> ANVWGVRLADSLSSPTIETRTRQYTLHDLCSDLDANPGREPWKPLRNQRTNNIVAVQLFRPLQGLVLDTQLYGFPGAFDDWERFMREKLRVLKYEVLRIYPISNYSNEHVNVFVANALVGAFLSNQAFYDLLPLLIINDTMIGDLLGTGASLSQFFQSHGDVLEVAAGRKYLQMENYSNDDDDPPLFAKDLSDYAKAFYSDTYEVLDRFFWTHDSSAGVLVHYDKPTNGHHYLLGTLTQMVSAPPYIINATDAMLLESCLEQFSANVRARPAQPVTRLDQCYHLRWGAQYVGEDSLTYRLGVLSLLATNGYQLARPIPRQLTNRWLSSFVSQIMSDGVNETPLWPQERYVQIAYDSPSVVDGATQYGYVRKNQLRLGMRISALQSLSDTPSPVQWLPQYTIDQAAMDEGDLMVSRLTQLPLRPDYGNIWVGDALSYYVDYNRSHRVVLSSELPQLPDTYFDGDEQYGRSLFSLARKIGDRSLVKDTAVLKHAYQAIDPNTGKEYLRSRQSVAYFGASAGHSGADQPLVIEPWIQGKISGVPPPSSVRQFGYDVARGAIVDLARPFPSGDYQFVYSDVDQVVDGHDDLSISSGLVESLLSSCMHATAPGGSFVVKINFPTRPVWHYIEQKILPNITSYMLIKPFVTNNVELFFVAFGVHQHSSLTWTSGVYFFLVDHFYRYETLSTISRQLPSFGYVDDGSSVTGIETISIENPGFSNMTQAARIGISGLCANVGNARKSIAIYESHGARVLTITSRRSPASARRKSRLRYLPLIDPRSLEVQARTILPADPVLFENVSGASPHVCLTMMYNFEVSSAVYDGDVVLDLGTGPEAKILELIPATSPVTCVDIRPTAQPSGCWNVRTTFLELDYLSDGWITGVRGDIVTCMLSLGAAAAGKSMTFDAAFQQLIKVLSKSTANVVLVQVNCPTDVVRSIKGYLEIDSTNKRYRFPKFGRDEPYSDMDALEKICRTAWPNCSITWVPLSYDLR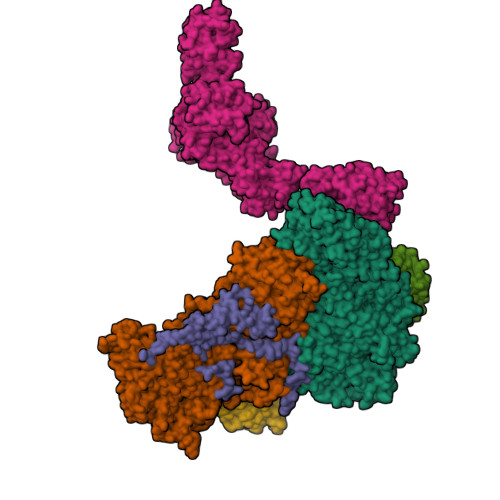WTRLALLESTTLSSASIRIAELMYKYMPIMRIDIHGLPMEKRGNFIVGQNCSLVIPGFNAQDVFNCYFNSALAFSTEDVNAAMIPQVSAQFDATKGEWTLDMVFSDAGIYTMQALVGSNANPVSLGSFVVDSPDVDITDAWPAQLDFTIAGTDVDITVNPYYRLMTFVRIDGQWQIANPDKFQFFSSASGTLVMNVKLDIADKYLLYYIRDVQSRDVGFYIQHPLQLLNTITLPTNEDLFLSAPDMREWAVKESGNTICILNSQGFVLPQDWDVLTDTISWSPSIPTYIVPPGDYTLTPL;>[3x]MKRIPRKTKGKSSGKGNDSTERADDGSSQLRDKQNNKAGPATTEPGTSNREQYKARPGIASVQRATESAEMPMKNNDEGTPDKKGNTKGDLVNEHSEAKDEADEATKKQAKDTDKSKAQVTYSDTGINNANELSRSGNVDNEGGSNQKPMSTRIAEATSAIVSKHPARVGLPPTASSGHGYQCHVCSAVLFSPLDLDAHVASHGLHGNMTLTSSDIQRHITEFISSWQNHPIVQVSADVENKKTAQLLHADTPRLVTWDAGLCTSFKIVPIVPAQVPQDVLAYTFFTSSYAIQSPFPEAAVSRIVVHTRWASNVDFDRDSSVIMAPPTENNIHLFKQLLNTETLSVRGANPLMFRANVLHMLLEFVLDNLYLNRHTGFSQDHTPFTEGANLRSLPGPDAEKWYSIMYPTRMGTPNVSKICNFVASCVRNRVGRFDRAQMMNGAMSEWVDVFETSDALTVSIRGRWMARLARMNINPTEIEWALTECAQGYVTVTSPYAPSVNRLMPYRISNAERQISQIIRIMNIGNNATVIQPVLQDISVLLQRISPLQIDPTIISNTMSTVSESTTQTLSPASSILGKLRPSNSDFSSFRVALAGWLYNGVVTTVIDDSSYPKDGGSVTSLENLWDFFILALALPLTTDPCAPVKAFMTLANMMVGFETIPMDNQIYTQSRRASAFSTPHTWPRCFMNIQLISPIDAPILRQWAEIIHRYWPNPSQIRYGAPNVFGSANLFTPPEVLLLPIDHQPANVTTPTLDFTNELTNWRARVCELMKNLVDNQRYQPGWTQSLVSSMRGTLDKLKLIKSMTPMYLQQLAPVELAVIAPMLPFPPFQVPYVRLDRDRVPTMVGVTRQSRDTITQPALSLSTTNTTVGVPLALDARAITVALLSGKYPPDLVTNVWYADAIYPMYADTEVFSNLQRDMITCEAVQTLVTLVAQISETQYPVDRYLDWIPSLRASAATAATFAEWVNTSMKTAFDLSDMLLEPLLSGDPRMTQLAIQYQQYNGRTFNIIPEMPGSVIADCVQLTAEVFNHEYNLFGIARGDIIIGRVQSTHLWSPLAPPPDLVFDRDTPGVHIFGRDCRISFGMNGAAPMIRDETGLMVPFEGNWIFPLALWQMNTRYFNQQFDAWIKTGELRIRIEMGAYPYMLHYYDPRQYANAWNLTSAWLEEITPTSIPSVPFMVPISSDHDISSAPAVQYIISTEYNDRSLFCTNSSSPQTIAGPDKHIPVERYNILTNPDAPPTQIQLPEVVDLYNVVTRYAYETPPITAVVMGVP;>ARAAFLFKTVGFGGLQNVPINDELSSHLLRAGNSPWQLTQFLDWISLGRGLATSALVPTAGSRYYQMSCLLSGTLQIPFRPNHRWGDIRFLRLVWSAPTLDGLVVAPPQVLAQPALQAQADRVYDCDDYPFLARDPRFKHRVYQQLSAVTLLNLTGFGPISYVRVDEDMWSGDVNQLLMNYFGHTFAEIAYTLCQASANRPWEYDGTYARMTQIVLSLFWLSYVGVIHQQNTYRTFYFQCNRRGDAAEVWILSCSLNHSAQIRPGNRSLFVMPTSPDWNMDVNLILSSTLTGCLCSGSQLPLIDNNSVPAVSRNIHGWTGRAGNQLHGFQVRRMVTEFCDRLRRDGVMTQAQQNQVEALADQTQQFKRDKLETWAREDDQYNQAHPNSTMFRTKPFTNAQWGRGNTGATSAAIAALI[2x]(2~{S},3~{R},4~{R},5~{S},6~{R})-5-fluoranyl-6-(hydroxymethyl)oxane-2,3,4-triol | C6 H11 F O5 | 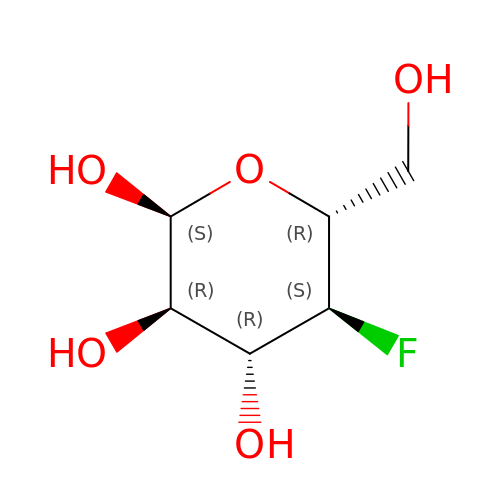FIHYONSINSKFAH-DVKNGEFBSA-N>[4x]HMQKVEVFRIPTASPDDISGLATLIDSGKINPAEIVAIL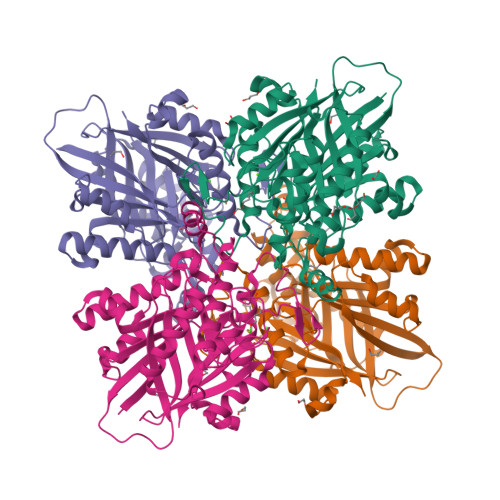GKTEGNGCVNDFTRGFATQSLAMYLAEKLGISREEVVKKVAFIMSGGTEGVMTPHITVFVRKDVAAPAAPGKRLAVGVAFTRDFLPEELGRMEQVNEVARAVKEAMKDAQIDDPRDVHFVQIKCPLLTAERIEDAKRRGKDVVVNDTYKSMAYSRGASALGVALALGEISADKISNEAICHDWNLYSSVASTSAGVELLNDEIIVVGNSTNSASDLVIGHSVMKDAIDADAVRAALKDAGIRSDDEMDRIVNVLAKAEAASSGTVRGRRNTMLDDSDINHTRSARAVVNAVIASVVGDPMVYVSGGAEHQGPDGGGPIAVIARV> QTDENRCLKANAKSCGECIQAGPNCGWCTNS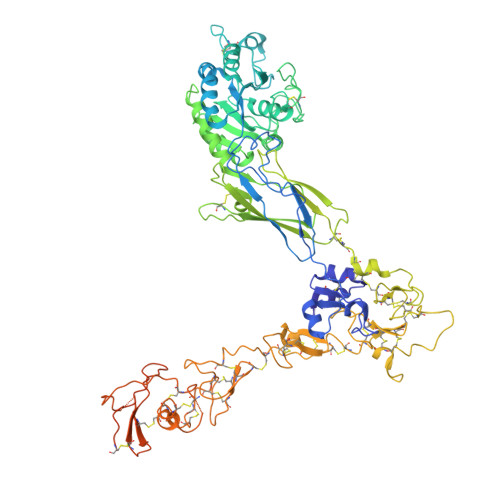TFLQEGMPTSARCDDLEALKKKGCPPDDIENPRGSKDIKKNKNVTNRSKGTAEKLKPEDIHQIQPQQLVLRLRSGEPQTFTLKFKRAEDYPIDLYYLMDLSYSMKDDLENVKSLGTDLMNEMRRITSDFRIGFGSFVEKTVMPYISTTPAKLRNPCTSEQNCTTPFSYKNVLSLTNKGEVFNELVGKQRISGNLDSPEGGFDAIMQVAVCGSLIGWRNVTRLLVFSTDAGFHFAGDGKLGGIVLPNDGQCHLENNMYTMSHYYDYPSIAHLVQKLSENNIQTIFAVTEEFQPVYKELKNLIPKSAVGTLSANSSNVIQLIIDAYNSLSSEVILENGKLSEGVTISYKSYCKNGVNGTGENGRKCSNISIGDEVQFEISITSNKCPKKDSDSFKIRPLGFTEEVEVILQYICECECQSEGIPESPKCHEGNGTFECGACRCNEGRVGRHCECSTDEVNSEDMDAYCRKENSSEICSNNGECVCGQCVCRKRDNTNEIYSGKFCECDNFNCDRSNGLICGGNGVCKCRVCECNPNYTGSACDCSLDTSTCEASNGQICNGRGICECGVCKCTDPKFQGQTCEMCQTCLGVCAEHKECVQCRAFNKGEKKDTCTQECSYFNITKVESRDKLPQPVQPDPVSHCKEKDVDDCWFYFTYSVNGNNEVMVHVVENPECPTGPDIIPIVAGVVAGIVLIGLALLLIWKLLMIIHDRREFAKFEKEKMNAKWDTGENPIYKSAVTTVVNPKYEGK>GLENIAFNVVKQGHFIGVEGELPVAVVNDKIFTKSGVNDICMFENKTTLPTNIAFELYAKRAVRSHPDFKLLHNLQADICYKFVLW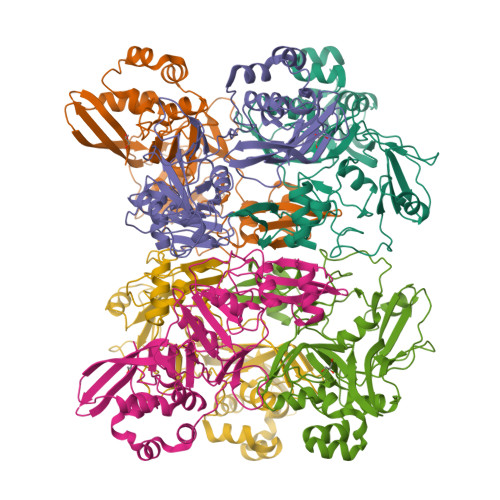DYERSNIYGTATIGVCKYTDIDVNSALNICFDIRDNCSLEKFMSTPNAIFISDRKIKKYPCMVGPDYAYFNGAIIRDSDVVKQPVKFYLYKKVNNEFIDPTECIYTQSRSCSDFLPLSDMEKDFLSFDSDVFIKKYGLENYAFEHVVYGDFSHTTLGGLHLLIGLYKRQQEGHIIMEEMLKGSSTIHNYFITETNTAAFKAVCSVIDLKLDDFVMILKSQDLGVVSKVVKVPIDLTMIEFMLWCKDGQVQTFYPRLQ[2x]> HGFVDNATIGGQFYQFYQPYQDPYMGSPPDRISRKIPGNGPVEDVTSLAIQCNADSAPAKLHASA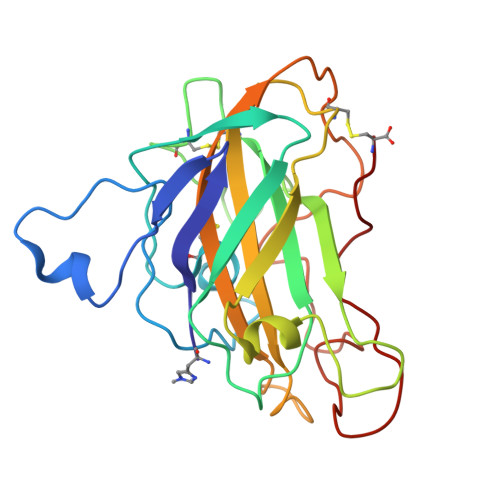AAGSTVTLRWTIWPDSHVGPVITYMARCPDTGCQDWTPSASDKVWFKIKEGGREGTSNVWAATPLMTAPANYEYAIPSCLKPGYYLVRHEIIALHSAYSYPGAQFYPGCHQLQVTGSGTKTPSSGLVSFPGAYKSTDPGVTYDAYQAATYTIPGPAVFTC>[2x]MEPAMEPETLEARINRATNPLNKELDWASINGFCEQLNEDFEGPPLATRLLAHKIQSPQEWEAIQALTVLETCMKSCGKRFHDEVG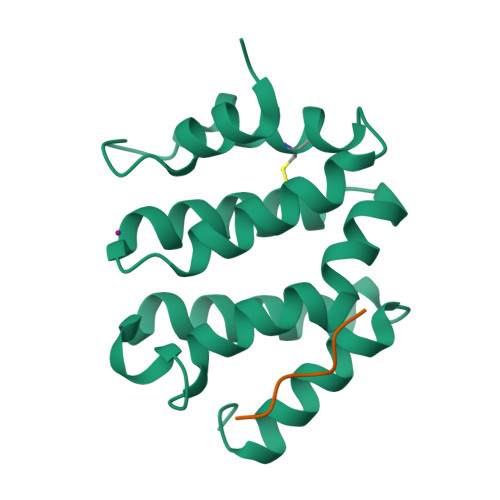KFRFLNELIKVVSPKYLGSRTSEKVKNKILELLYSWTVGLPEEVKIAEAYQMLKKQGIVKS;>SFHDDSDEDLLHI[2x]>[2x]PKHEFSVDMTCGGCAEAVSRVLNKL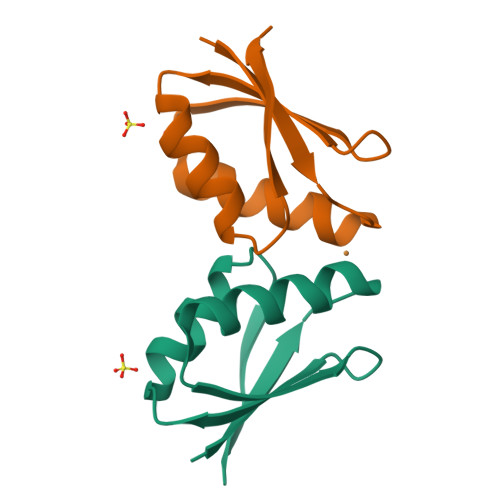GGVKYDIDLPNKKVCIESEHSMDTLLATLKKTGKTVSYLGLE>MHHHHHHSETSRTAFGGRRAVPPNNSNAAEDDLPTVELQGVVPRGVNLQEFLNVTSVHLFKERWDTNKVDHHTDKYENNKLIVRRGQSFYVQIDFSRPYDPRRDLFRVEYVIGRYPQENKGTYIPVPIVSELQSGKWGAKIVMREDRSVRLSIQSSPKCIVGKFRMYVAVWTPYGVLRTSRNPETDTYILFNPWCEDDAVYLDNEKEREEYVLNDIGVIFYGEVNDIKTRSWSYGQFEDGILDTCLYVMDRAQMDLSGRGNPIKVSRVGSAMVNAKDDEGVLVGSWDNIYAYGVPPSAWTGSVDILLEYRSSENPVRYGQCWVFAGVFNTFLRCLGIPARIVTNYFSAHDNDANLQMDIFLEEDGNVN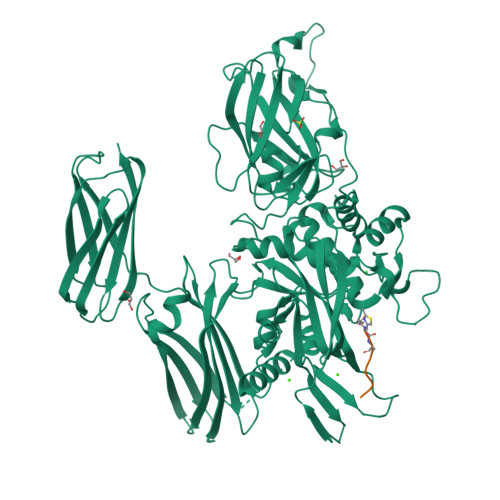SKLTKDSVWNYHCWNEAWMTRPDLPVGFGGWQAVDSTPQENSDGMYRCGPASVQAIKHGHVCFQFDAPFVFAEVNSDLIYITAKKDGTHVVENVDATHIGKLIVTKQIGGDGMMDITDTYKFQEGQEEERLALETALMYGAKKPLNTEGVMKSRSNVDMDFEVENAVLGKDFKLSITFRNNSHNRYTITAYLSANITFYTGVPKAEFKKETFDVTLEPLSFKKEAVLIQAGEYMGQLLEQASLHFFVTARINETRDVLAKQKSTVLTIPEIIIKVRGTQVVGSDMTVIVEFTNPLKETLRNVWVHLDGPGVTRPMKKMFREIRPNSTVQWEEVCRPWVSGHRKLIASMSSDSLRHVYGELDVQIQRRPSM[2x]>[3x]GSHMVNIIQKFIPVGANNRPGYAMKPKYITVHNTANTAVGADAAAHARYLKNPDTTTSWHFTVDDKEIYQHLPLNENGWHAGDGNGSGNRASIGIEICENADGDFAKATANAQWLIK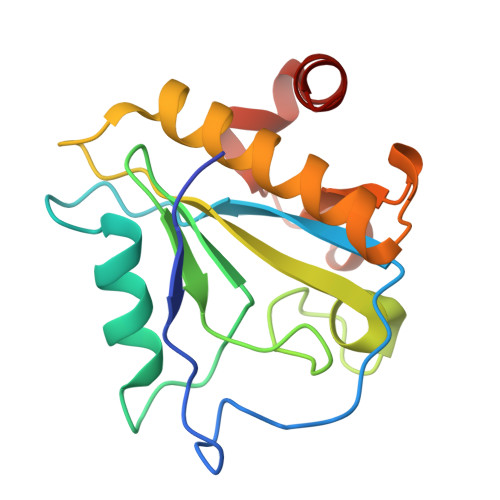TLMAEHNISLANVVPHKYWSGKECPRKLLDKWDSFKAGIG> MDNVDFAESVRTRWARRLIREKVAKE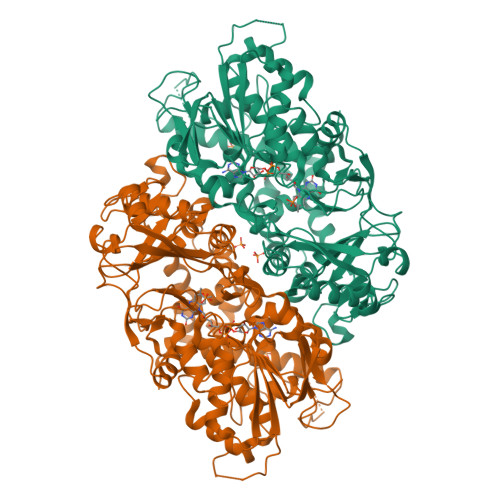LNILTERLGEVPGIPPPREGRFLGGGYSHDNLPSDPLYSSIKPALLKEAPRAEEELPPRKVCIVGAGVSGLYIAMILDDLKIPNLTYDIFESSSRTGGRLYTHHFTDAKHDYYDIGAMRYPDIPSMKRTFNLFKRTGMPLIKYYLDGENTPQLYNNHFFAKGVVDPYMVSVANGGTVPDDVVDSVGEKLQQAFGYYKEKLAEDFDKGFDELMLVDDMTTREYLKRGGPKGEAPKYDFFAIQWMETQNTGTNLFDQAFSESVIDSFDFDNPTKPEWYCIEGGTSLLVDAMKETLVHKVQNNKRVEAISIDLDAPDDGNMSVKIGGKDYSGYSTVFNTTALGCLDRMDLRGLNLHPTQADAIRCLHYDNSTKVALKFSYPWWIKDCGITCGGAASTDLPLRTCVYPSYNLGDTGEAVLLASYTWSQDATRIGSLVKDAPPQPPKEDELVELILQNLARLHAEHMTYEKIKEAYTGVYHAYCWANDPNVGGAFALFGPGQFSNLYPYLMRPAAGGKFHIVGEASSVHHAWIIGSLESAYTAVYQFLYKYKMWDYLRLLLERWQYGLQELETGKHGTAHLQFILGSLPKEYQVKI>[4x]SMDKSTDDTSKVTYFVTLEREGDEKIVLEKGQPFVEPGYYAEMNGEDITESVQIKGSVDVNTPGIYNLVYAAYNEDGFAKTFTRTVYVADNTASPLKSGIYTVAE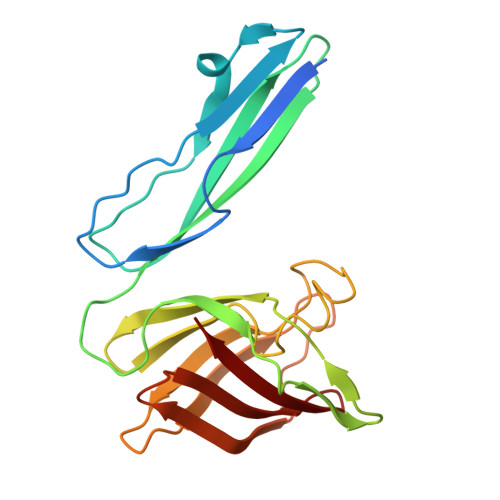GSKRTAPSVVAFSGYEIVIFQMEPGIFYISDFLGGWYDQRAGYGPDYAMVGKFELNDDNTITPLESYVAGWGDSMDQMTNTLLDPATGTLKWTVAYAGQLSFDIIVKQ> MKKFYRLLGSSSVALLGCLFLSVALCIAEEAEGVKGVAEEEL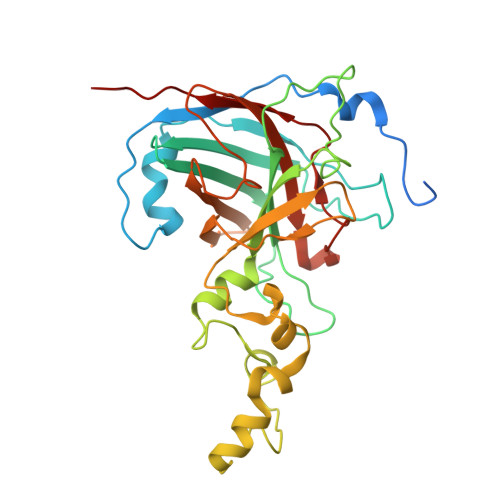TPAKEVLNVKYMQIDVPAHITVGALEGAFKNAEGVQVKLQKQDKAFPNGGGSVNSAEIKAIHDGITIYFQVIWDDATDNKQAIATQEFRDGAALMFPLGKITISPEEPFSPRMGDRQKPVNLWHWKADWEADLLATGGIEECPARYPNMHDDFSTNPHSVNYHKGVIQSAAELSGGYAAHNLLSLPRGRAVEDLNAEGFGTLTSQDHQDVDGCSKFENKKWTVVFCRSLNTGDPLDVQFVPGESTYFNMAVWNGDREDRNGQKNISIQWHPLSLERIAWQ>[6x]GMADFQ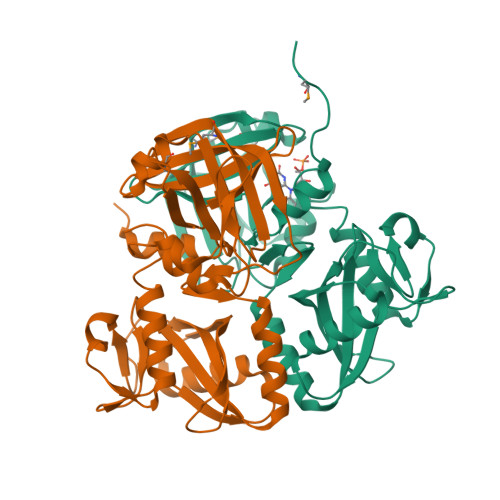GETEMTAEVFDPRALRDAFGAFATGVTVVTASDAAGKPIGFTANSFTSVSLDPPLLLVCLAKSSRNYESMTSAGRFAINVLSETQKDVSNTFARPVEDRFAAVDWRLGRDGCPIFSDVAAWFECSMQDIIEAGDHVIIIGRVTAFENSGLNGLGYARGGYFTPRLAGKAVSAAVEGEIRLGAVLEQQGAVFLAGNETLSLPNCTVEGGDPARTLAAYLEQLTGLNVTIGFLYSVYEDKSDGRQNIVYHALASDGAPRQGRFLRPAELAAAKFSSSATADIINRFVLESSIGNFGIYFGDETGGTVHPIANKDAHS> GIGTGFPFDPHYVEVLGERMHYVDVGPRDGTPVLFLHGNPTSSYVWRNIIPHVAPTHRCIAPDLIGMGKSDKPDLGYFFDDHVRFMDAFIEALGLEEVVLVIHDWGSALGFHWAKRNPERVKGIAFMEFIRPIPTWDEWPEFARETFQAFRTTDVGRKLIIDHNVFIEGTLLMGVVRPLTEVEMDHYREPFLNPVDREPLWRFPNELPIAGEPANIVALVEEYMDWLHQSPVPKLLFWG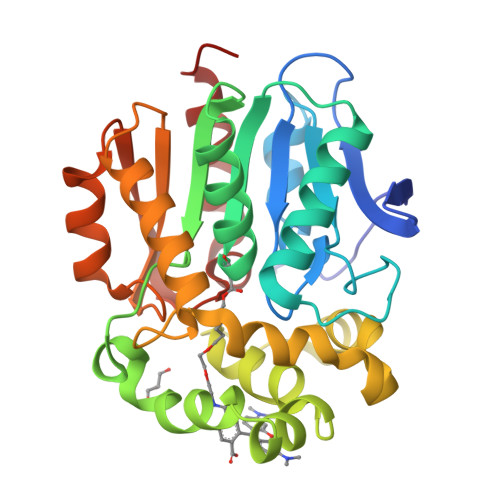TPGVLIPPAEAARLAKSLPNCKAVDIGPGLNLLQEDNPDLIGSEIARWLSTLEI>GSAACEPVRIPLCKSLPWEMTKMPNHLHHSTQANAILAMEQFE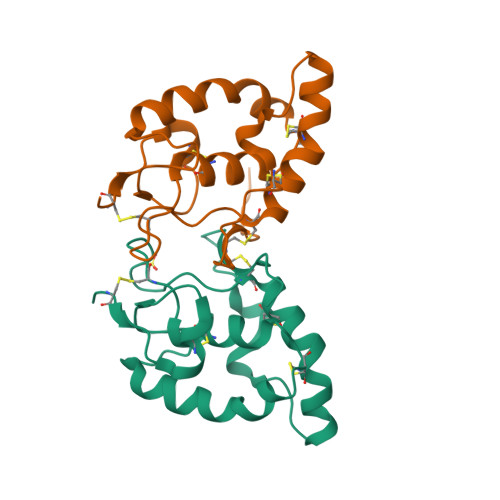GLLGTHCSPDLLFFLCAMYAPICTIDFQHEPIKPCKSVCERARQGCEPILIKYRHSWPESLACDELPVYDRGVCISPEAIVTAD[6x]> PISPIETVPVKLKPGMDGPKVKQWPLTEEKIKALVEICTEMEKEGKISKIGPENPYNTPVFAIKKKDSTKWRKLVDFRELNKRTQDFWEVQLGIPHPAGLKKKKSVTVLDVGDAYFSVPLDEDFRKYTAFTIPSINNKT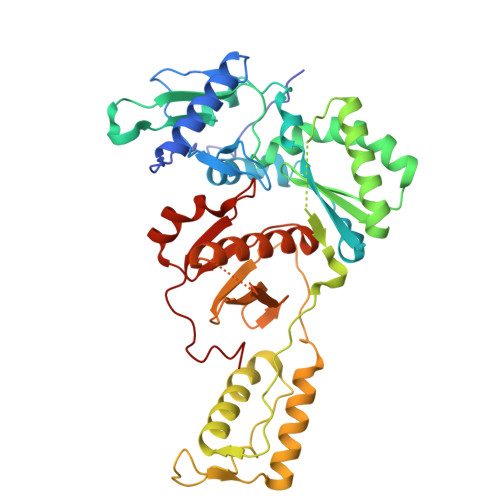PGIRYQYNVLPQGWKGSPAIFQSSMTKILEPFKKQNPDIVIYQYMDDLYVGSDLEIGQHRTKIEELRQHLLRWGLTTPDKKHQKEPPFLWMGYELHPDKWTVQPIVLPEKDSWTVNDIQKLVGKLNWASQIYPGIKVRQLSKLLRGTKALTEVIPLTEEAELELAENREILKEPVHGVYYDPSKDLIAEIQKQGQGQWTYQIYQEPFKNLKTGKYARMRGAHTNDVKQLTEAVQKITTESIVIWGKTPKFKLPIQKETWETWWTEYWQATWIPEWEFVNTPPLVKLWYQ>[2x]GSMSTINFANREINFKIVYYGPGLSGKTTNLKWIYSKVPEGRKGEMVSLATEDERTLFFDFLPLDIGEVKGFKTRFHLYTVPGQVFYNASRKLILRGVD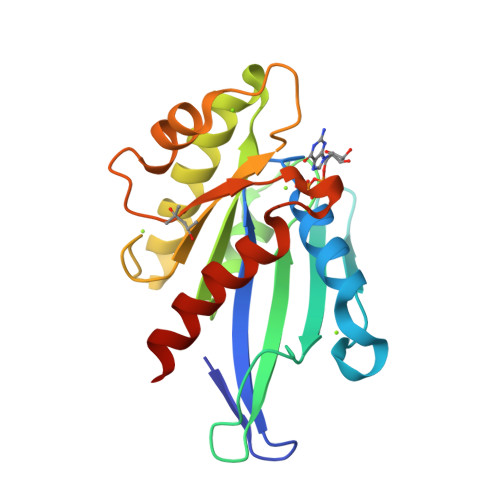GIVFVADSAPNRLRANAESMRNMRENLAEYGLTLDDVPIVIQVNKRDLPDALPVEMVRAVVDPEGKFPVLEAVATEGKGVFETLKEVSRLVLARVAGGS> CPRF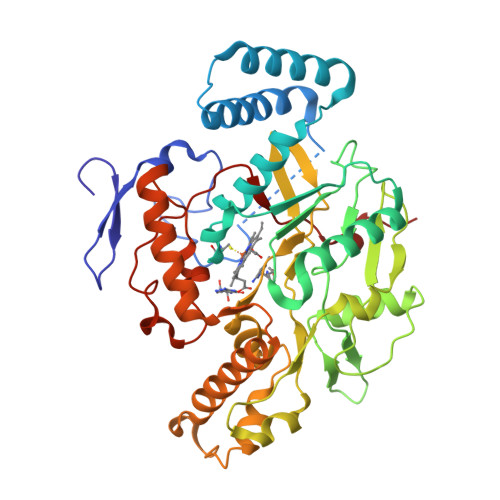LKVKNWETDVVLTDTLHLKSTLETGCTEHICMGSIMLPSQHTRKPEDVRTKDQLFPLAKEFLDQYYSSIKRFGSKAHMDRLEEVNKEIESTSTYQLKDTELIYGAKHAWRNASRCVGRIQWSKLQVFDARDCTTAHGMFNYICNHVKYATNKGNLRSAITIFPQRTDGKHDFRVWNSQLIRYAGYKQPDGSTLGDPANVQFTEICIQQGWKAPRGRFDVLPLLLQANGNDPELFQIPPELVLEVPIRHPKFDWFKDLGLKWYGLPAVSNMLLEIGGLEFSACPFSGWYMGTEIGVRDYCDNSRYNILEEVAKKMDLDMRKTSSLWKDQALVEINIAVLYSFQSDKVTIVDHHSATESFIKHMENEYRCRGGCPADWVWIVPPMSGSITPVFHQEMLNYRLTPSFEYQPDPWNTHVWKG> PDYVFHRAHERMLFQTSYTLENNGSVICIPNNGQCFCLAWLKSNGTNAEKLAANILQWITFALSALCLMFYGYQTWKSTCGWEEIYVATIEMIKFIIEYFHEFDEPAVIYSSNGNKTVWLRYAEWLLTCPVILIHLSNLTGLANDYNKRTMGLLVSDIGGIVWATTAALSKGYVRVIFFLMGLCYGIYTFFNAAKVYIEAYHTVPKGRCRQVVTGMAWLFFVSWGMFPILFILGPEGFGVLSVYGSTVGHTIIDLMSKNCWGLLGHYLRVLIHEHILIHGDIRKTTKLNIGGTEIEVETLVEDE

One of the major families of such protein tools consists of microbial opsins, membrane proteins characterized by seven transmembrane helices that bind a chromophore, retinal, to a lysine residue of the protein through a protonated Schiff base linkage, RPSB3. In optogenetics, some microbial opsins such as channelrhodopsins (ChRs) and archaerhodopsin-3 (AR3), which function as light-sensitive ion transporters, are heterologously expressed in animal neurons to excite and silence them, and consequently to control animal behaviours by illumination with light. In the present study, we rationally develop largely blue-shifted colour variants of microbial rhodopsins, using theoretical chemistry, biochemistry, electrophysiology and X-ray crystallography. We introduced point mutations that enforce torsion around the C6–C7 bond from planarity in C1C2 and AR3, to shrink the π-conjugation and consequently to produce blue shifts of their absorption spectra328.

The T198G/G202A mutant of C1C2 (C1C2GA) showed a blue-shifted absorption spectrum (λmax=455 nm) as compared with that of wild-type C1C2 (C1C2WT; λmax=476 nm), which was well predicted by the torsion at the C6–C7 bond. The atomistically designed structural model that created the blue-shifted spectrum was verified by solving the crystal structure of the C1C2GA mutant. We expressed, purified and crystallized C1C2GA as previously described24, and obtained yellow crystals in the lipidic cubic phase under neutral pH conditions (pH 7.0). As expected, the overall structure of C1C2GA at pH 7.0 is almost identical to that of C1C2WT at pH 6.0 (root mean squared deviation of 0.66 Å over all Cα atoms), except for the protonation states of titratable groups, the amino-terminal (N-terminal) segment, and the retinal-binding pocket. In contrast to C1C2WT, the electron density of C1C2GA clearly indicated the rotation of the β-ionone ring. The space where the C17 methyl group resides in C1C2WT becomes occupied by the methyl group of the alanine residue introduced by the mutation, and instead the C17 methyl group occupies the pocket formed by the threonine to glycine mutation. The C5=C6–C7=C8 dihedral angle changes from 177.7° to −31.4° (counterclockwise, positive), and consequently the retinal configuration changes from 6-s-trans to 6-s-cis. The atomic resolution structure is in good agreement with the calculated model, and it strongly supports the present design principle that the simultaneous double mutations at positions 198 and 202 in C1C2 (118 and 122 in HsBR, respectively) induce the rotation of the β-ionone ring, which leads to the significant blue-shift of the absorption spectrum. Notably, Asp40, His44 and His47 on the N-terminal helix coordinate a cation with Asp142 on ECL1. Owing to the strong electron density and the tetrahedral coordination by the His and Asp residues, this cation is most likely an endogenous Zn2+ ion.> KLITASSSKEYLPDLLLFWQNYEYWITNIGLYKTKQRDLTRTPANLDTDTEECMFWMNYLQKDQSFQLMNFAMENLGALYFGSIGDISELYLRVEQYWDRRADKNHSVDGKYWDALIWSVFTMCIYYMPVEKLAEIFSVYPLHEYLGSNKRLNWEDGMQLVMCQNFARCSLFQLKQCDFMAHPDIRLVQAYLILATTTFPYDEPLLANSLLTQCIHTFKNFHVDDFRPLLNDDPVESIAKVTLGRIFYRLCGCDYLQSGPRKPIALHTEVSSLLQHAAYLQDLPNVDVYREENSTEVLYWKIISLDRDLDQYLNKSSKPPLKTLDAIRRELDIFQYKVDSLEEDFRSNNSRFQKFIALFQISTVSWKLFKMYLIYYDTADSLLKVIHYSKVIISLIVNNFHAKSEFFNRHPMVMQTITRVVSFISFYQIFVESAAVKQLLVDLTELTANLPTIFGSKLDKLVYLTERLSKLKLLWDKVQLLDSGDSFYHPVFKILQNDIKIIELKNDEMFSLIKGLGSLVPLNKLRQESLLEEE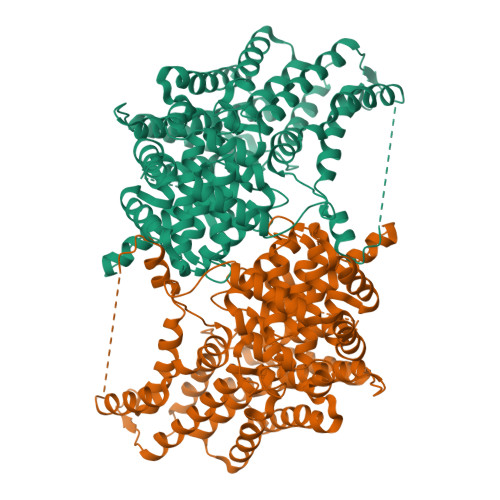DENNTEPSDFRTIVEEFQSEYNISDILS>[3x]GSNLVAQLENEVASLENENETLKKKNLHKKDLIAYLEKEIANLRKKI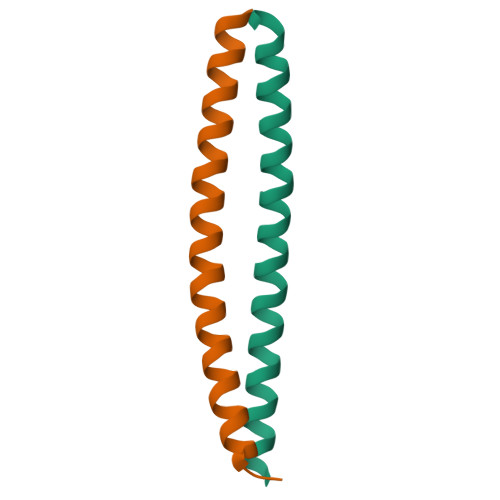EE;>[3x]GSARNAYLRKKIARLKKDNLQLERDEQNLEKIIANLRDEIARLENEVASHEQ>[4x]RFTPLGIDEFYIKPCERKIVYTTDKHDKCLMRRLEIEMDTGENQGYVKCVFKEFGYLNGEGQFNKQALLKDYHQAGFKNKDKAVLESYDGCMKNYG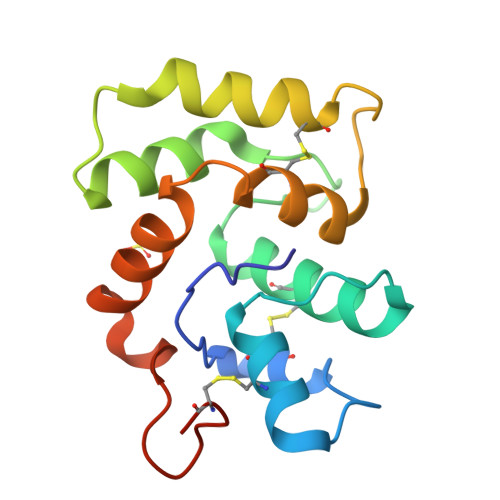PTPNAMKILDCVTKDKDFPKVINARRERNSDWKPDWIQAYCGVTKLF(2S)-2-[(2-azanyl-4-oxidanylidene-3H-pteridin-7-yl)carbonylamino]-3-(4-hydroxyphenyl)propanoic 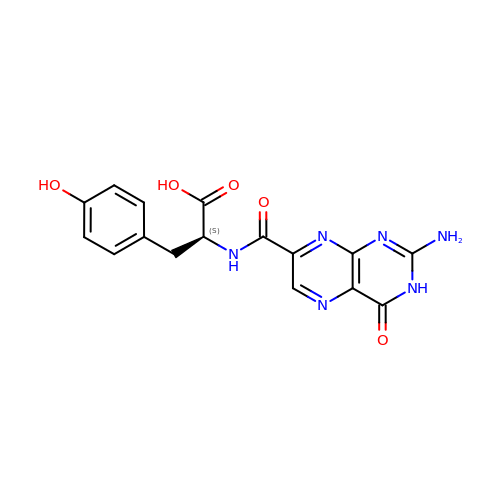acid | C16 H14 N6 O5 | BYYDVPCOJAQWPZ-VIFPVBQESA-N>HHHHHHSSGLVPRGSHMHFTIQREALLKPLQLVAGVVERRQTLPVLSNVLLVVEGQQLSLTGTDLEVELVGRVVLEDAAEPGEITVPARKLMDICKSLPNDVLIDIRVEEQKLLVKAGRSRFTLSTLPANDFPTVE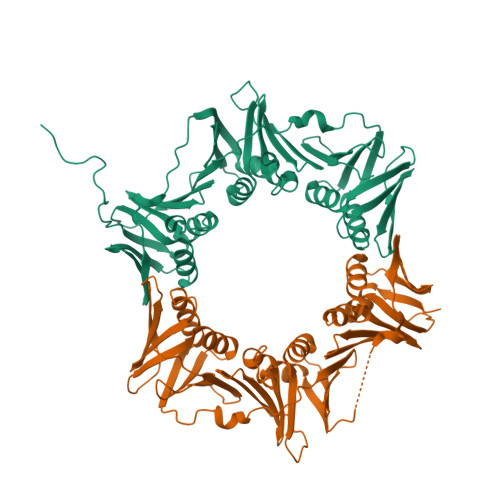EGPGSLNFSIAQSKLRRLIDRTSFAMAQQDVRYYLNGMLLEVNGGTLRSVATDGHRLAMCSLDAQIPSQDRHQVIVPRKGILELARLLTEQDGEVGIVLGQHHIRATTGEFTFTSKLVDGKFPDYERVLPRGGDKLVVGDRQQLREAFSRTAILSNEKYRGIRLQLSNGLLKIQANNPEQEEAEEEVQVEYNGGNLEIGFNVSYLLDVLGVIGTEQVRFILSDSNSSALVHEADNDDSAYVVMPMRL[2x]>[2x]MGSSRTMTVDTGEEL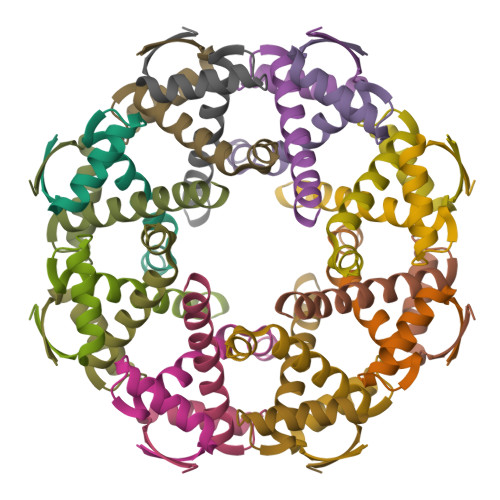RAFVEGLVESGDYKTNSEVIRDGLRLLQEKTAGSKLAALRLEHHHHHH>MTPASYNLAVRRAAPAVVNVYNRGLNTNSHNQLEIRTLGSGVIMDQRGYIITNKHVINDADQIIVALQDGRVFEALLVGSDSLTDLAVLKINATGGLPTIPINARRVPHIGDVVLAIGNPYNLGQTITQGIISATGRIGLNPTGRQNFLQTDASINHGNSGGALVNSLGELMGINTLSFDKSNDGETPEGIGFAIPFQLATKIMDKLIRDGRVIRGYIGIGGREIAPLHAQGGGIDQLQGIVVNEVSPDGPAANAGIQVNDLIISVDNKPAISALET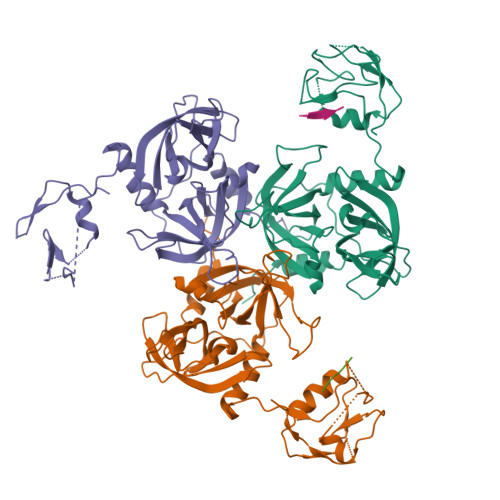MDQVAEIRPGSVIPVVVMRDDKQLTLQVTIQEYPATN[3x];>DNRLGLVYQF[2x]The mitotic kinase MASTL (microtubule-associated serine/threonine kinase-like) - more commonly known as Greatwall kinase or GWL - belongs to the AGC family of serine/threonine protein kinases and has recently emerged as a potential target for cancer chemoprevention. GWL exerts its biological activity by phosphorylating α-endosulfine (ENSA) and/or cAMP-regulated phosphoprotein 19 (ARPP19). Once phosphorylated, these proteins become potent inhibitors of the protein phosphatase 2A complex (PP2A/B55). Negative regulation of PP2A/B55 by GWL thus results in a positive feedback loop that boosts CDK1 activity above the threshold required for mitotic entry.

Although highly related at the amino acid sequence level to the N- and C-terminal kinase lobes of the MAST kinases (microtubule-associated serine/threonine kinase; MAST1, 2, 3 and 4) and other AGC kinases, GWL has a highly unusual architecture, with an ~500 amino acid insertion between the DFG and APE motifs of the activation segment connecting the N- and C-terminal lobes (NCMR; non-conserved middle region). We therefore excised the NCMR of hGWL and replaced it with four amino acids 496 - RTFC - 499 taken from human PKCα, to generate the expression construct ‘hGWL-KinDom’ (see Experimental Section). Diffracting crystals of hGWL-KinDom in complex with STU were obtained from commercially available screens. The structure was determined by molecular replacement, and refined at a resolution of 3.1Å (Figure S3 and Table S1 for crystallographic and refinement data). As expected, hGWL-KinDom adopts the classical ‘two-lobe’ protein kinase domain fold. As both the C-helix and activation loop regions are disordered in electron density maps, this strongly suggests that just the non-phosphorylated form of hGWL-KinDom (in complex with STU) was selectively incorporated into protein crystals. As expected, STU occupies the nucleotide-binding pocket, making hydrogen bonds to the backbone carbonyl and nitrogen of hinge residues Glu111 and Leu113, via its lactam nitrogen (N6) and oxygen (O6) groups, respectively (nomenclature as described in [31]). It is also ‘sandwiched’ on both sides, by several hydrophobic residues, including Ile41, Val49, Ala60 and Leu163 from the N-lobe, and Thr173 and Leu163 from the C-lobe. In electron density maps, we can observe amino acids 825-854 of the GWL C-terminal extension, containing both the C-lobe anchor (CLA) and the majority of the C-lobe tether (CLT) motifs (bottom). As in other AGC-kinases, such as PDK1 and PKCα, the GWL C-terminal extension wraps across one face of the C-lobe, making an extensive series of predominantly hydrophobic interactions.

>[2x]GPHMDPTAGSKKEPGGGAATEEGVNRIAVPKPPSIEEFSIVKPISRGAFGKVYLGQKGGKLYAVKVVKKADMINKNMTHQVQAERDALALSKSPFIVHLYYSLQSANNVYLVMEYLIGGDVKSLLHIYGYFDEEMAVKYISEVALALDYLHRHGIIHRDLKPDNMLISNEGHIKLTDFGLSKVTLNRDINMMDILTTRTFCGTPDYLAPELLLGRAHGPAVDWWALGVCLFEFLTGIPPFNDETPQQVFQNILKRDIPWPEGEEKLSDNAQSAVEILLTIDDTKRAGMKELKRHPLFSDVDWENLQHQTMPFIPQPDDETDTSYFEARNTAQHLTVSGFSL> MKKLLNTLYVTQPDTYLSLDGDNVVLLKEQEKLGRLPLHNLEAIVGFGYTGASPALMGYCAERNISITFLTKNGRFLARVVGESRGNVVLRKTQYRISENDQESTKIARNFITGKVYNSKWMLERMTREHPLRVNVEQFKATSQLLSVMMQEIRNCDSLESLRGWEGQAAINYNKVFDQMILQQKEEFAFHGRSRRPPKDNVNAMLSFAYTLLANDVAAALETVGLDAYVGFMHQDRPGRASLALDLMEELRGLYADRFVLSLINRKEMTADGFYKKENGAVLMTDEARKTFLKAWQTKKQEKITHPYLGEKMSWGLVP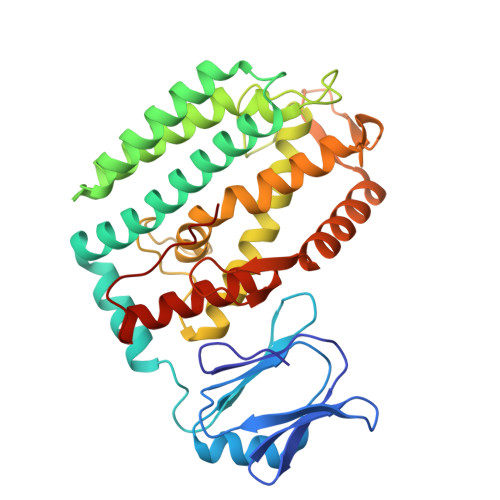YVQALLLARFLRGDLDEYPPFLWK> MGSSHHHHHHSSGLVPRGSHSDEVDAHMTTNTVSRKVAWLRVVTLAVAAFIFNTTEFVPVGLLSDIAQSFHMQTAQVGIMLTIYAWVVALMSLPFMLMTSQVERRKLLICLFVVFIASHVLSFLSWSFTVLVISRIGVAFANAIFWSITASLAIRMAPAGKRAQALSLIATGTALAMVLGLPLGRIVGQYFGWRMTFFAIGIGALITLLCLIKLLPLLPSEHSGSLKSLPLLFRRPALMSIYLLTVVVVTAHYTAYSYIEPFVQNIAGFSANFATALLLLLGGAGIIGSVIFGKLGNQYASALVSTAIALLLVCLALLLPAANSEIHLGVLSIFW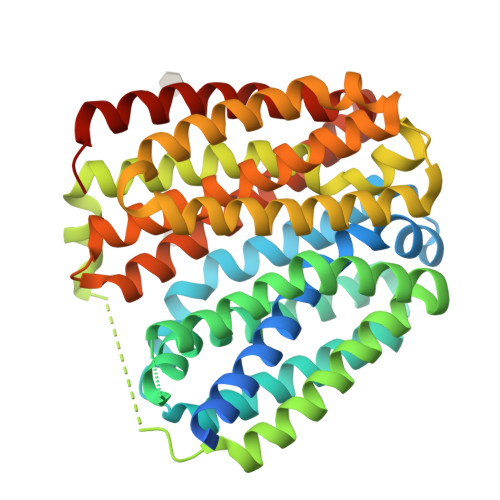GIAMMIIGLGMQVKVLALAPDATDVAMALFSGIFNIGIGAGALVGNQVSLHWSMSMIGYVGAVPAFAALIWSIIIFRRWPVTLEEQTQ Ferritin from the marine pennate diatom Pseudo-nitzschia multiseries (PmFTN) plays a key role in sustaining growth in iron-limited ocean environments. Typically formed from 24 subunits arranged as a symmetric, hollow sphere, ferritins take up soluble Fe2+ and catalyze its oxidation, with the resulting Fe3+ being stored as an oxy-hydroxide mineral in its central cavity. The di-iron catalytic ferroxidase center of PmFTN (sites A and B) has a nearby third iron site (site C) in an arrangement typically observed in prokaryotic ferritins. Here we demonstrate that Glu-44, a site C ligand, and Glu-130, a residue that bridges iron bound at sites B and C, limit the rate of post-oxidation reorganization of iron coordination and the rate at which Fe3+ exits the ferroxidase center for storage within the mineral core.

Glu-130, a ligand that can coordinate iron at both site B and site C, was substituted with the non-coordinating residue alanine. Two structures were obtained from E130A PmFTN crystals soaked for 5 min (E130A Fe (5 min)) and overnight (E130A Fe (o.n.)) in aerobic Fe2+ solutions, respectively. In the E130A Fe (o.n.) structure, iron was found in binding sites A, B, and C. Iron occupancy at site A was 50–60%, whereas in site B, iron was observed in only six of eight subunits with an occupancy of 15–35%. Fe-C has an occupancy of 40–65%. The iron coordination spheres of Fe-A and Fe-C are as in the wild type protein, except for the absence of the Glu-130 side chain. As seen in the E44Q Fe (45 min) structure (data not shown), Asn-97 is coordinated to Fe-B in the E130A Fe (o.n.) structure. In addition to these sites, up to two iron ions with occupancies of 40–55% were found beyond site C toward the mineral core, as seen in wild type PmFTN. One iron ion is coordinated by Glu-47, and the other is coordinated by Glu-44 and solvent molecules. Substitution of the site B/C coordinating residue Glu-130 with alanine, a non-coordinating residue, led to a striking 10-fold increase in mineralization activity; this is unusual in that active site mutations rarely enhance activity.

>[8x]GSEELLDLFNRQVTQEFTASQVYLSASIWFDQNDWEGMAAYMLAESAEEREHGLGFVDFANKRNIPIELQAVPAPVSCAEWSSPEDVWQSILELEQANTRSLLNLAEAASTCHDFAVMAFLNPFHLQQVNAEDKIGSILAKVTDENRTPGLLRSLDVVSFLGPCLFRS>GHMTSRPSSDQTWQPIDGRVALIAPASAIATDVLEATLRQLEVHGVDYHLGRHVEARYRYLAGTVEQRLEDLHNAFDMPDITAVWCLRGGYGCGQLLPGLDWGRLQAASPRPLIGFSDISVLLSAFHRHGLPAIHGPVATGLGLSPLSAPREQQERLASLASVSRLLAGIDHELPVQHLGGHKQRVEGALIGGNLTALACMAGTLGGLHAPAGSILVLEDVGEPYYRLERSLWQLLESIDARQLGAICLGSFTDCPRKEVAHSLERIFGEYAAAIEVPLYHHLPSGHGAQNRAWP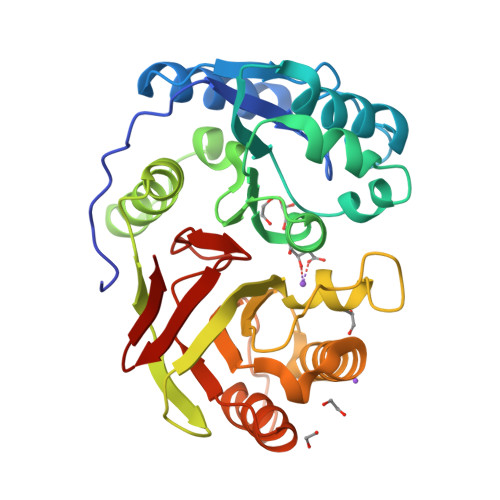YGKTAVLEGNRLRWGS[2x]>[2x]MNHKVHHHHHHIEGRHMKRLTYISKFSRPLSGDEIEAIGRISSQKNQQANVTGVLLCLDGIFFQILEGEAEKIDRIYERILADERHTDILCLKSEVEVQERMFPDWSMQTINLDENTDFLIRPIKVLLQTLTESHRILEKYTQPSIFKIISQGTNPLNIRPKAVEKIVFFSDIVSFSTFAEK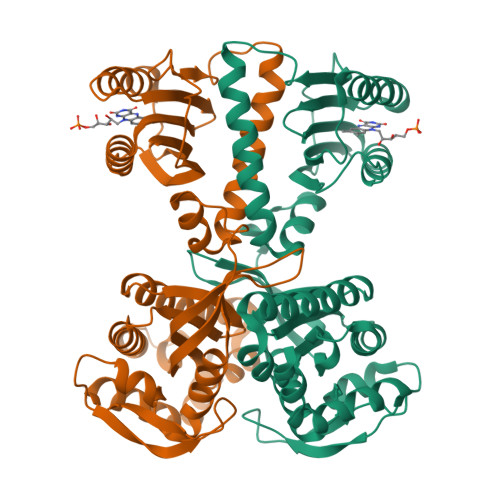LPVEEVVSVVNSYFSVCTAIITRQGGEVTKFIGDCVMAYFDGDCADQAIQASLDILMELEILRNSAPEGSPLRVLYSGIGLAKGKVIEGNIGSELKRDYTILGDAVNVAARLEALTRQLSQALVFSSEVKNSATKSWNFIWLTDSELKGKSESIDIYSIDNEMTRKSSGGLEIARNIGHYLERVGDRQPSQIFGVKSLPL>MGSSHHHHH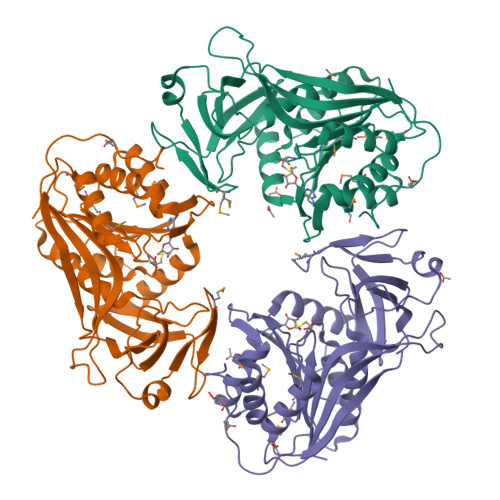HSSGRENLYFQGMQRTGELPAEHVPVILESSGAGDFHLIDSGNGLKLEQYGDYRVVRPEAQALWRPLVPDRVWQNADAIFTGDTDEDGMGRWRFPKEALGETWPLSLLGVEFLGRFTAFRHVGVFPEQIVHWEWLKNAVETADRPLKVLNLFGYTGVASLVAAAAGAEVTHVDASKKAIGWAKENQVLAGLEQAPIRWICEDAMKFIQREERRGSTYDIILTDPPKFGRGTHGEVWQLFDHLPLMLDICREILSPKALGLVLTAYSIRASFYSMHELMRETMRGAGGVVASGELVIREAGLDGKTPGRVLSTSLFSRWEPKGS[3x]Protein complexes of the mitochondrial respiratory chain assemble into respiratory supercomplexes. Here we present the high-resolution electron cryo-microscopy structure of the Arabidopsis respiratory supercomplex consisting of complex I and a complex III dimer, with a total of 68 protein subunits and numerous bound cofactors. A complex I-ferredoxin, subunit B14.7 and P9, a newly defined subunit of plant complex I, mediate supercomplex formation. We propose that the main role of the plant supercomplex is to stabilize its components in the membrane.

The matrix channels at ND2 and ND4 seem to be closed under our experimental conditions, whereas the one of ND5 is open. One is located at the tip of the membrane arm at ND5. This half-channel has also been seen in complex I from mammals and Yarrowia lipolytica. In our structure, this channel is connected to the central aqueous passage while proton leakage from the open ND5 matrix half-channel is prevented by a 5–6 Å gap between ND5 H257 and T315. The B14.7/C1-FDX/lipid arrangement stabilizes this loop together with an amphipathic helix that runs towards the main ND5 transmembrane domain at the tip of the membrane arm.

> MYLLIVFLPLLGSSVAGFFGRFLGSEGSAIMTTTCVSFSSILSLIAFYEVALGASACYLRIAPWISSEMFDASWGFLFDSLTVVMLIVVTFISSLVHLYSISYMSEDPHSPRFMCYLSIFTFFMLMLVTGDNFLQLFLGWEGVGLASYLLIHFWFTRLQADKAAIKAMLVNRVGDFGLALGILGCFTLFQTVDFSTIFACASVPRNSWIFCNMRLNAISLICILLFIGAVGKSAQIGLHTWLPDAMEGPTPVSALIHAATMVTAGVFMIARCSPLFEYSPTALIVITFAGAMTSFLAATTGILQNDLKRVIAYSTCSQLGYMIFACGISNYSVSVFHLMNHAFFKALLFLSAGSVIHAMSDEQDMRKMGGLASSFPLTYAMMLIGSLSLIGFPFLTGFYSKDVILELAYTKYTISGNFAFWLGSVSVLFTSYYSFRLLFLTFLVPTNSFGRDISRCHDAPIPMAIPLILLALGSLFVGYLAKDMMIGLGTNFWANSLLVLPKNEILAESEFAAPTIIKLIPILFSTLGAFVAYNVNLVADQFQRAFQTSTFCNRLYSFFNKRWFFDQVLNDFLVRSFLRFGYEVSFEALDKGAIEILGPYGISYTFRRLAERISQLQSGFVYHYAFAMLLGLTLFVTFFCMWDSLSSWVDNRLSFILIVSSFYTKSSQE;> MLEHFCECYFNLSGLILCPVLGSIILLFIPNSRIRLIRLIGLCASLITFLYSLVLWIQFDSSTAKFQFVESLRWLPYENINFYLGIDGISLFFVILTTFLIPICILVGWSGMRSYGKEYIIAFLICEFLMIAVFCMLDLLLFYVFFESVLIPMFIIIGVWGSRQRKIKAAYQFFLYTLLGSLFMLLAILLILFQTGTTDLQILLTTEFSERRQIFLWIAFFASFAVKVPMVPVHIWLPEAHVEAPTAGSVILAGILLKFGTYGFLRFSIPMFPEATLCFTPFIYTLSAIAIIYTSLTTLRQIDLKKIIAYSSVAHMNLVTIGMFSLNIQGIGGSILLMLSHGLVSSALFLCVGVLYDRHKTRLVRYYGGLVSTMPNFSTIFFFFTLANMSLPGTSSFIGEFLILVGAFQRNSLVATLAALGMILGAAYSLWLYNRVVSGNLKPDFLHKFSDLNGREVFIFIPFLVGLVWMGVYPKVFLDCMHTSVSNLVQHGKFH;> MALRNAILRHLRVPVQTLGLNQSKIGFLGTIRSFSSHDDHLSREAVVDRVLDVVKSFPKVDPSKVTPEVHFQNDLGLDSLDTVEIVMAIEEEFKLEIPDKEADKIDSCSLAIEYVYNHPMSS;> MGGGDHGHGAEGGDFRAKVWSMTGGPNCRPKHWRRNTAIAMFGVFLVCIPIAKLSAKLEQRPHMPVRPIPSQIWCKNFGTKDDYEKEH;> MPSTQSLTVAAKTLRNRIFSRSGSTSAGPSRWATPGHEERPKGYFMNRTPPAPGQSRKWEDWELPCYITSFLTIVILGVGLNAKPDLSIETWAHQKALERLEMEKLATAGDSSD;> MGFIMEFAENLVLRLMENPEERDRKAREHIYEMHERCKKIKEMWALPIRPYGFWTFERHNAQLRWDPQISQVAGRRDPYDDLLEDNYTPPSSSSSSSD;> MGGGGHGGGITYKGVTVHTPKTWHTVTGKGLCAVMWFWILYRAKQDGPVVMGWRHPWDGHGDHGHGDHH;> MAKPLGTTGEFFRRRDEWRKHPMLSNQMRHALPGIGIGVGAFCVYLVGEQIYSKLMAPSSQSSHQKQPAPSH;> MAGRLSGVASRIMGGNGVVARSVGSSLRQRAGMGLPVGKHIVPDKPLSVNDELMWDNGTAFPEPCIDRIADTVGKYEALAWLSGGLGFFVGLGLLAVLNDKASKVPFTPRVYPYDNLRVELGGEP;> MGGGMETNKNKFIEDWGSARENLEHNFRWTRRNFALIGIFGIALPIIVYKGIVKDFHMQDEDAGRPHRKFL;> MSGVSTAAYFARRAAQKERVRILYRRALKDTLNWAVHRHIFYRDASDLREKFNVNQDVEDVDRIDKLIAHGEAEYNKWRHPDPYIVPWAPGGSKFCRNPTPPAGIEIVYNYGLEDNP;> MEVPGSSKKMIATQEEMSAAKIALGSRDMCAHLLIPLNKCRQAEFYLPWKCEDERHVYEKCEYELVMERMLAMKKIREEEALAKQNKLQGNAAVPLIPKTANA;> MGRKKGLPEFEESAPDGFDPENPYKDPVAMVEMREHIVREKWIQIEKAKILREKVKWCYRVEGVNHYQKCRHLVQQYLDSTRGVGWGKDHRPISLHGPKPEAVEAE> EGVSNLVGLPNNICLQKTSNQILKPKLISYTLPVVGQSGTCITDPLLAMDEGYFAYSHLERIGSCSRGVSKQRIIGVGEVLDRGDEVPSLFMTNVWTPPNPNTVYHCSAVYNNEFY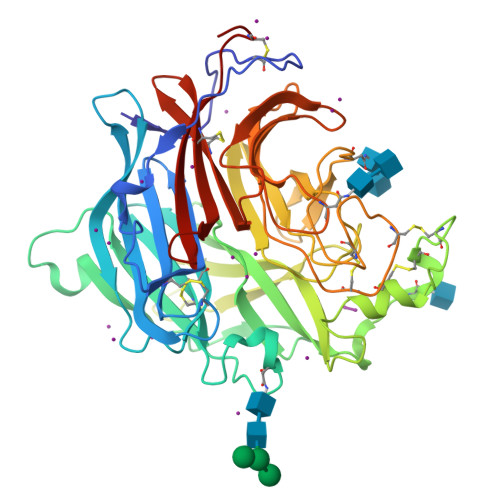YVLCAVSTVGDPILNSTYWSGSLMMTRLAVKPKSNGGGYNQHQLALRSIEKGRYDKVMPYGPSGIKQGDTLYFPAVGFLVRTEFKYNDSNCPITKCQYSKPENCRLSMGIRPNSHYILRSGLLKYNLSDGENPKVVFIEISDQRLSIGSPSKIYDSLGQPVFYQASFSWDTMIKFGDVLTVNPLVVNWRNNTVISRPGQSQCPRFNTCPEICWEGVYNDAFLIDRINWISAGVFLDSNQTAENPVFTVFKDNEILYRAQLASEDTNAQKTITNCFLLKNKIWCISLVEIYDTGDNVIRPKLFAVKIPEQCTA>SDKTEPRNEVYKDKFKNQYNSWHDTAKSEELVDALEQDPNMVILWAGYAFAKDYKAPRGHMYAVTDVRNTLRTGAPKNAEDGPLPMACWSCKSPDVPRLIEEQGEDGYFKGKWAKGGPEVTNTIGCSDCHEKGSPKLRISRPYVDRALDAIGTPFSKASKQDKESMVCAQCHVEYYFEKKEDKKGFVKFPWDMGVTVDQMEVYYDGIEFSDWTHALSKTPMLKAQHPEYETWKMGIHGKNNVSCVDCHMPKVTSP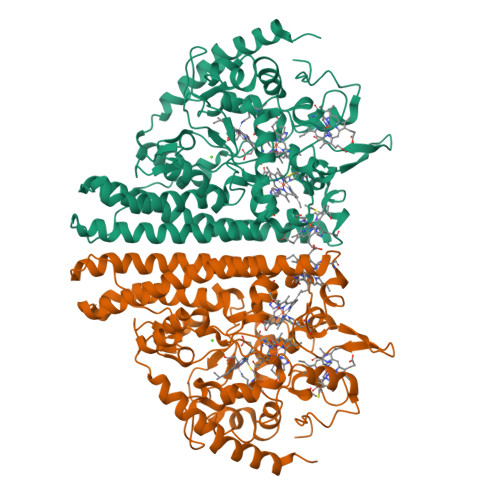EGKKFTDHKVGNPFDRFEETCATCHSQTKEFLVGVTNERKAKVKEMKLKAEEQLVKAHFEAAKAWELGATEAEMKPILTDIRHAQWRWDLAIASHGVAAHAPEEALRVLGTSVNKAADARVKLAQLLAKKGLTDPVAIPDISTKAKAQAVLGMDMEKMNAEKEAFKKDMLPKWDAEAKKREATY[2x]> QCDNFPQMLRDLRDAFSRVKTFFQTKDEVDNLL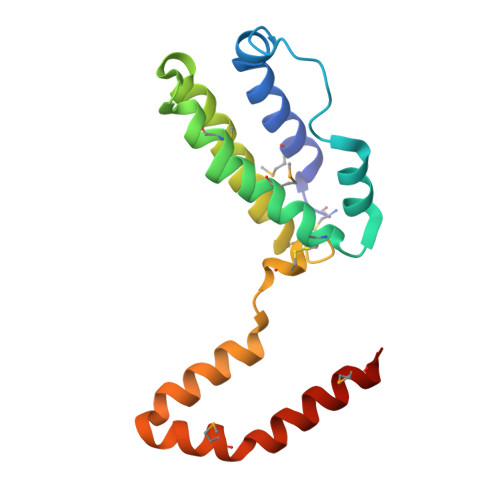LKESLLEDFKGYLGCQALSEMIQFYLEEVMPQAENQDPEIKDHVNSLGENLKTLRLRLRRCHRFLPCENKSKAVEQIKNAFNKLQEKGIYKAMSEFDIFINYIEAYMTIKAR1-[4-(1,2,3-thiadiazol-4-yl)phenyl]methanamine 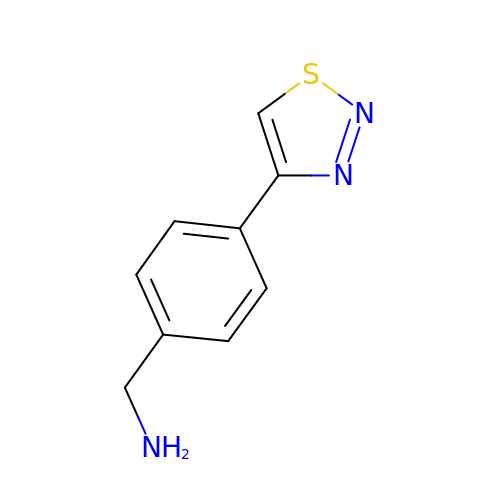| C9 H9 N3 S | FWSCINFUBQNPJM-UHFFFAOYSA-N>MAAATGPSFWLGNETLKVPLALFALNRQRLCERLRKNPAVQAGSIVVLQGGEETQRYCTDTGVLFRQESFFHWAFGVTEPGCYGVIDVDTGKSTLFVPRLPASHATWMGKIHSKEHFKEKYAVDDVQYVDEIASVLTSQKPSVLLTLRGVNTDSGSVCREASFDGISKFEVNNTILHPEIVECRVFKTDMELEVLRYTNKISSEAHREVMKAVKVGMKEYELESLFEHYCYSRGGMRHSSYTCICGSGENSAVLHYGHAGAPNDRTIQNGDMCLFDMGGEYYCFASDITCSFPANGKFTADQKAVYEAVLRSSRAVMGAMKPGVWWPDMHRLADRIHLEELAHMGILSGSVDAMVQAHLGAVFMPHGLGHFLGIDVHDVGGYPEGVERIDEPGLRSLRTARHLQPGMVLTVEPGIYF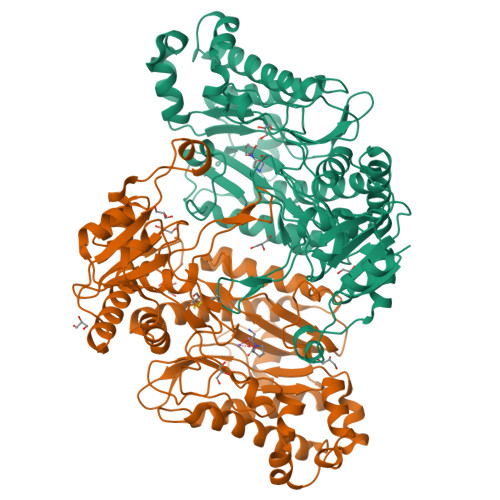IDHLLDEALADPARASFLNREVLQRFRGFGGVRIEEDVVVTDSGIELLTCVPHTVEEIEACMAGCDKAFTPFSGPK[2x]>[6x]MGKACLQNGTRLLRADGSEVLVEDVQEGDQLLGPDG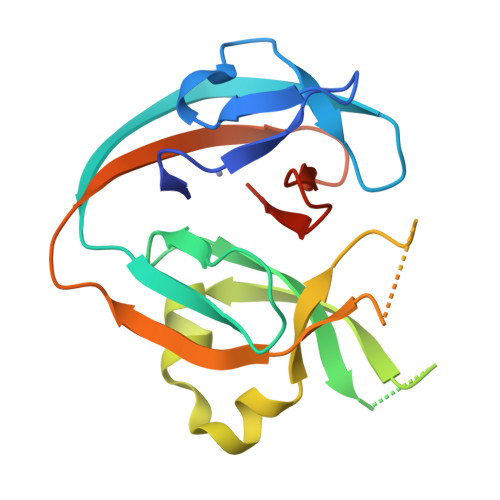TSRTASKIVRGEERLYRIKTHEGLEDLVCTHNHILSMYKERFGREGAHSPSAGTSLTESHERVDVTVDDFVRLPQQEQQKYKLFRSTDFVRREQPSASKLATLLHINSIELEEEPTKWSGFVVDKDSLYLRYDYLVLHNSLEHHHHHH>GSHMSDLPLRFPYGRPEFLGLSQDEVEASADHIARPILILKETRRLPWATGYAEVINAGKSTHNEDQASCEVLTVKKKAGAVTSTPNRNSSKRRSSLPNGEGLQLKENSESEGVSCHYWSLFDGHAGSGAAVVASRLLQHHITEQLQD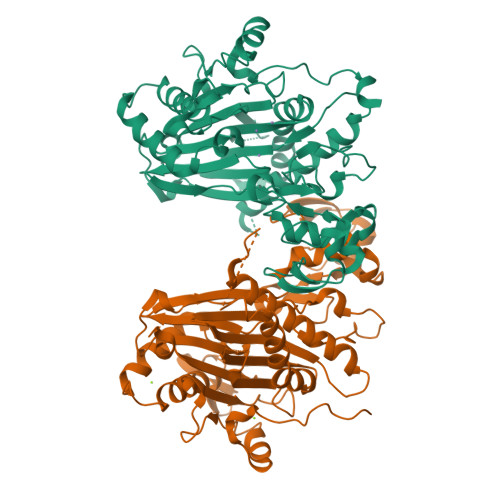IVDILKNSAVLGSGSTRFFTEKKIPHECLVIGALESAFKEMDLQIERERSSYNISGGCTALIVICLLGKLYVANAGDSRAIIIRNGEIIPMSSEFTPETERQRLQYLAFMQPHLLGNEFTHLEFPRRVQRKELGKKMLYRDFNMTGWAYKTIEDEDLKFPLIYGEGKKARVMATIGVTRGLGDHDLKVHDSNIYIKPFLSSAPEVRIYDLSKYDHGSDDVLILATDGLWDVLSNEEVAEAITQFLPNCDPDDPHRYTLAAQDLVMRARGVLKDRGWRISNDRLGSGDDISVYVIPLIHGNKLS[2x]>[3x]MMVISEKVRKA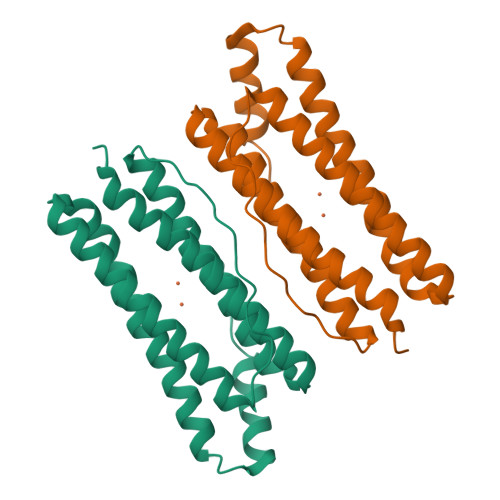LNDQLNREIYSSYLYLSMATYFDAEGFKGFAHWMKKQAQEELTHAMKFYEYIYERGGRVELEAIEKPPSNWNGIKDAFEAALKHEEFVTQSIYNILELASLALDHATVSFLKWFVDEQVEEEDQVLEILDLLEKAFGQMSVIFQLDRYLGQRE>MRTELLSKLYDDFGIDQLPHTQHGVTSDRLGKLYEKYILDIFKDIESLKKYNTNAFPQEKDISSKLLKALNLDLDNIIDVSSSDTDLGRTIAGGSPKTDATIRFTFHNQSSRLVPLNIKHSSKKKVSIAEYDVETICTGVGISDGELKELIRKHQNDQSAKLFTPVQKQRLTELLEPYRERFIRWCVTLRAEKSEGNILHPDLLIRFQVIDREYVDVTIKNIDDYVSDRIAEGSKARKPGFGTGLNWTYASGSKAKKMQFKG[2x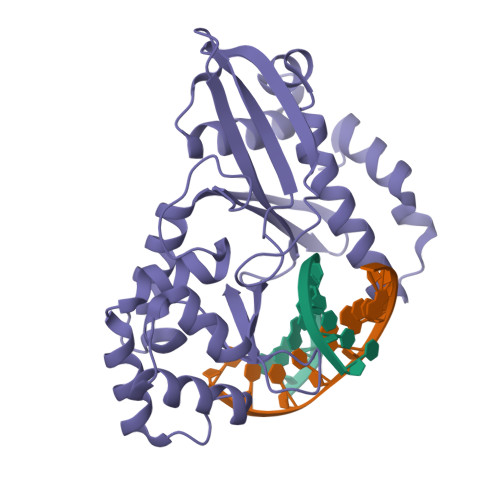]3-butyl-1-(2,2-diphosphonoethyl)pyridinium 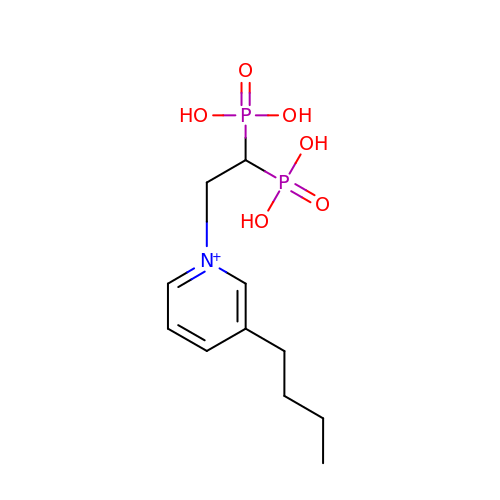| C11 H20 N O6 P2 | QVWIHYAQHVVJSB-UHFFFAOYSA-O> SGRGKG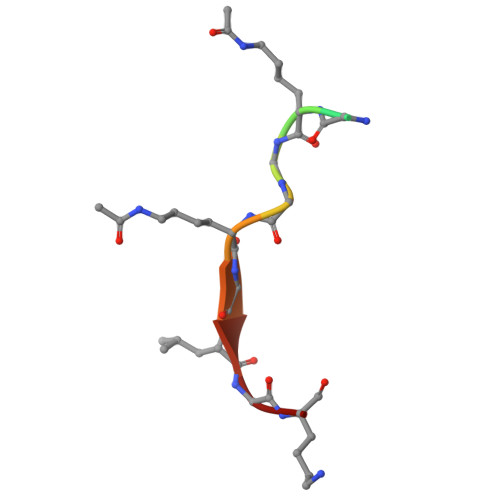GKGLGK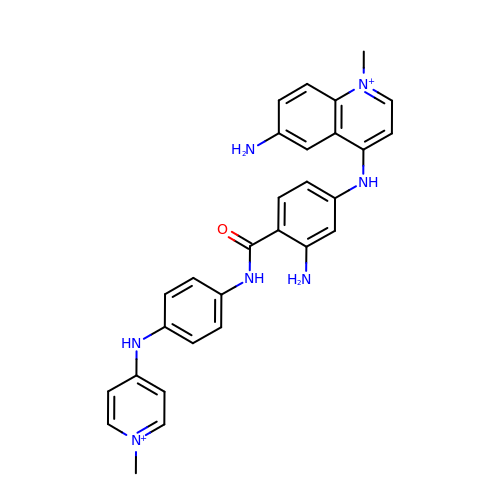4-[4-[2-AMINO-4-[4,6-(N-METHYLQUINOLINIUM)AMINO]BENZAMIDO]ANILINO]-N-METHYLPYRIDINIUM MESYLATE | C29 H29 N7 O | DOZAHXWWOPAJKW-UHFFFAOYSA-P> PHLVIEATANLRLETSPGELLEQANKALFASGQFGEADIKSRFVTLEA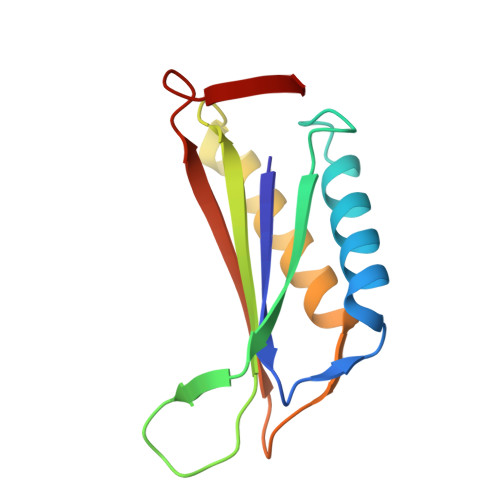YRQGTAAVERAYLHACLSILDGRDIATRTLLGASLCAVLAEAVAGGGEEGVQVSVEVREMERLSYAKRVV> MKFYIDDLPVLFPYPKIYPEQYNYMCDIKKTLDVGGNSILEMPSGTGKTVSLLSLTIAYQMHYPEHRKIIYCSRTMSEIEKALVELENLMDYRTKELGYQEDFRGLGLTSRKNLCLHPEVSKERKGTVVDEKCRRMTNGQAKRKLEEDPEANVELCEYHENLYNIEVEDYLPKGVFSFEKLLKYCEEKTLCPYFIVRRMISLCNIIIYSYHYLLDPKIAERVSNEVSKDSIVIFDEAHNIDNVCIESLSLDLTTDALRRATRGANALDERISEVRKVDSQKLQDEYEKLVQGLHSADILTDQEEPFVETPVLPQDLLTEAIPGNIRRAEHFVSFLKRLIEYLKTRMKVLHVISETPKSFLQHLKQLTFIERKPLRFCSERLSLLVRTLEVTEVEDFTALKDIATFATLISTYEEGFLLIIEPYEIENAAVPNPIMRFTCLDASIAIKPVFERFSSVIITSGTISPLDMYPRMLNFKTVLQKSYAMTLAKKSFLPMIITKGSDQVAISSRFEIRNDPSIVRNYGSMLVEFAKITPDGMVVFFPSYLYMESIVSMWQTMGILDEVWKHKLILVETPDAQETSLALETYRKACSNGRGAILLSVARGKVSEGIDFDHQYGRTVLMIGIPFQYTESRILKARLEFMRENYRIRENDFLSFDAMRHAAQCLGRVLRGKDDYGVMVLADRRFSRKRSQLPKWIAQGLSDADLNLSTDMAISNTKQFLRTMAQPTDPKDQEGVSVWSYEDLIKHQNSRKDQGGFIENENKEGEQDEDEDEDIEMQ;> MSHSGAAIFEKVSGIIAINEDVSPAELTWRSTDGDKVHTVVLSTIDKLQATPASSEKMMLRLIGKVDESKKRKDNEGNEVVPKPQRHMFSFNNRTVMDNIKMTLQQIISRYKDADIYEEKRRREESAQHTETPMSSSSVTAGTPTPHLDTPQLNNGAPLINTAKLDDSLSKEKLLTNLKLQQSLLKGNKVLMKVFQETVINAGLPPSEFWSTRIPLLRXFALXXSQKXGPXXVXXXXXPXXXXXXXXXXNLSREKILNIFENYPIVKKAYTDNVPKNFKEPEFWARFFSSKLFRKLXXXXXXXXXXXXXXXXXXLXXXXXFXXKXXXXLLHPVKKIIXLDGNIXDDPVVRGXXXXXXXXVDILKGMNRLSEKMIMXLKXXXXXXXXXXXXXXXXXXXXXXXXXXXXXXXXXXXXXXXXRVITXIKINAKQAXHXXXEVKSTLPIDLLESCRMLHTTCCEFLKHFAIHQKQASTVKKLYNHLKDCIEKLNELFQDVLNGDGESMSNTCTAYLKPVLNSITLATHKYDEYFNEYNNNSN;> MSDYSLKHSVTQYLEEIPQQVQNRLYTSPATCLAIYRILPPLAKFFIMAMVFNENEVPLLDLDKWVNSNGKLQFQNAIKSMKSLHLLIPNKSSGTLMINLNPTFKISLRNALTGGEVQNSFGVVVEENVVSLDLLDEYSANKWETILHFMVGTPLAKIPSEKVLNLLKHSKLMEEVNSTGEFKITNEGFQFLLQEINSQLWTLLLQYLKMIETSKMDLVDVLHFIFMLGALEVGKAYKIDALSETQRIMLQDMRDYGLVFQKHSNDSIFYPTKLALMLTSDTKTIRSASNAMDSVLRQNREEPSVNEDGANGKSTTDITTSDDLNKAGLKNQDIPDGSLIVETNFKIYSYSNSPLQIAVLSLFVHLKARFVNMVLGQITRESIRRALTNGITADQIIAYLETHAHPQMRRLAEEKLEKKLELDPNCKEPLQVLPPTVVDQIRLWQLELDRVITYEGSLYSDFETSQEYNLLSKYAQDIGVLLWKDDKKKKFFISKEGNSQVLDFAKRKLKKKQ;> MLMDEYEENKDMCPICKTDRYLSPDVKFLVNPECYHRICESCVDRIFSLGPAQCPYKGCDKILRKNKFKTQIFDDVEVEKEVDIRKRVFNVFNKTIDDFNGDLVEYNKYLEEVEDIIYKLDHGIDVAKTEEKLRTYEELNKQLIMNNLERSRTEIESFEQRQKFEKEMKLKKRLLERQIEEEERMNKEWTKKEIVNRLSTTTQDINETIEGVKNTVKLKKSSARRKLEELNRVLKNNPYFNSNVNVQNSRLKDAVPFTPFNGDREAHPRFTLKGSVYNDPFIKDLEHRKEFIASGFNTNYAYERVLTEAFMGLGCVISEEL;> MDAISDPTFKHARSRKQVTEESPSLLTVIIEIA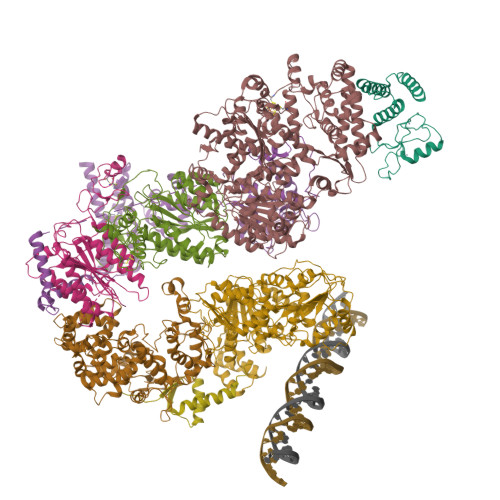PKLWTTFDEEGNEKGSIIKVLEALIVFLNAHLAFNSANKVAVIAAYSQGIKYLYPESTSALKASESENKTRSDLKIINSXXYRRFRNVDETLVEEIYKLFELEKKQIEQNSQRSTLAGAMSAGLTYVNRISKESVTTSLKSRLLVLTCGSGSSKDEIFQYIPIMNCIFSATKMKCPIDVVKIGGSKESTFLQQTTDATNGVYLHVESTEGLIQYLATAMFIDPSLRPIIVKPNHGSVDFRTSCYLTGRVVAVGFICSVCLCVLSIIPPGNKCPACDSQFDEHVIAKLKRKPVVPRLKAKKKVTKP;> MARARKGALVQCDPSIKALILQIDAKMSDIVLEELDDTHLLVNPSKVEFVKHELNRLLSKNIYNPMDEEENQ;> MAPVVISESEEDEDRVAITRRTKRQVHFDGEGDDRVDQQQQQHSSSHRDRDKHVQRKKKKRLSNRNLQGSNGGYAWEDEIKRSWDLVKVDDEGDMASLVASIVEARKKRTAKKNITPYQRGIIRSLILTLDCSEAMLEKDLRPNRHAMIIQYAIDFVHEFFDQNPISQMGIIIMRNGLAQLVSQVSGNPQDHIDALKSIRKQEPKGNPSLQNALEMARGLLLPVPAHCTREVLIVFGSLSTTDPGDIHQTIDSLVSEKIRVKVLGLSAQVAICKELCKATNYGDESFYKILLDETHLKELFNEAVTPLPVNKINKGFTLVKMGFPTRIFEDTPTFCSCHSKLVYGGYFCPNCHSKVCSLPTVCPCCDLMLILSTHLARSYHHLMPLKTFAEVPTTEKFRSEDCFSCQSRFPXXXXXXXXXXXXXSRYRCEDCKQEFCVDCDVFIHEILHNCPGCESKPVIT;> MTDVEGYQPKSKGKIFPDMGESFFSSDEDSPATDAEIDENYDDNRETSEGRGERDTGAMVTGLKKPRKKTKSSRHTAADSSMNQMDAKDKALLQDTNSDIPADFVPDSVSGMFRSHDFSYLRLRPDHASRPLWISPSDGRIILESFSPLAEQAQDFLVTIAEPISRPSHIHEYKITAYSLYAAVSVGLETDDIISVLDRLSKVPVAESIINFIKGATISYGKVKLVIKHNRYFVETTQADILQMLLNDSVIGPLRIDSDHQVQPPEDVLQQQLQQTAGKPATNVNPNDVEAVFSAVIGGDNEREEEDDDIDAVHSFEIANESVEVVKKRCQEIDYPVLEEYDFRNDHRNPDLDIDLKPSTQIRPYQEKSLSKMFGNGRARSGIIVLPCGAGKTLVGITAACTIKKSVIVLCTSSVSVMQWRQQFLQWCTLQPENCAVFTSDNKEMFQTESGLVVSTYSMVANTRNRSHDSQKVMDFLTGREWGFIILDEVHVVPAAMFRRVVSTIAAHAKLGLTATLVREDDKIGDLNFLIGPKLYEANWMELSQKGHIANVQCAEVWCPMTAEFYQEYLRETARKRMLLYIMNPTKFQACQFLIQYHERRGDKIIVFSDNVYALQEYALKMGKPFIYGSTPQQERMNILQNFQYNDQINTIFLSKVGDTSIDLPEATCLIQISSHYGSRRQEAQRLGRILRAKRRNDEGFNAFFYSLVSKDTQEMYYSTKRQAFLVDQGYAFKVITHLHGMENIPNLAYASPRERRELLQEVLLKNEEAAGIEVGDDADNSVGRGSNGHKRFKSKAVRGEGSLSGLAGGEDMAYMEYSTNKNKELKEHHPLIRKMYYKNLKK>MTHVEVVATITPQLSIEETLIQKINHRIDAIDVLELRIDQFENVTVDQVAEMITKLKVMQDSFKLLVTYRTKLQGGYGQFTNDSYLNLISDLANINGIDMIDIEWQADIDIEKHQRIITHLQQYNKEVIISHHNFESTPPLDELQFIFFKMQKFNPEYVKLAVMPHNKNDVLNLLQAMSTFSDTMDCKVVG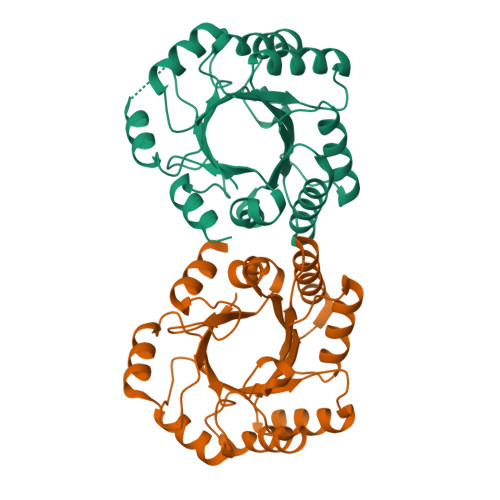ISMSKLGLISRTAQGVFGGALTYGCIGEPQAPGQIDVTDLKAQVTLY[2x]> MPTLLRVYIDGPHGMGKTTTTQLLVALGSRDDIVYVPEPMTYWRVLGASETIANIYTTQHRLDQGEISAGDAAVVMTSAQITMGMPYAVTDAVLAPHIGGEAGSSHAPPPALTLIFDRHPIAALLCYPAARYLMGSMTPQAVLAFVALIPPTLPGTNIVLGALPEDRHIDRLAKRQRPGERLDLAMLAAIRRVYGLLANTVRYLQCGGSWREDWGQLSGTAVPPQGAEPQSNAGARPHIGDTLFTLFRAPELLAPNGDLYNVFAWALDVLAKRLRSMHVFILDYDQSPAGCRDALL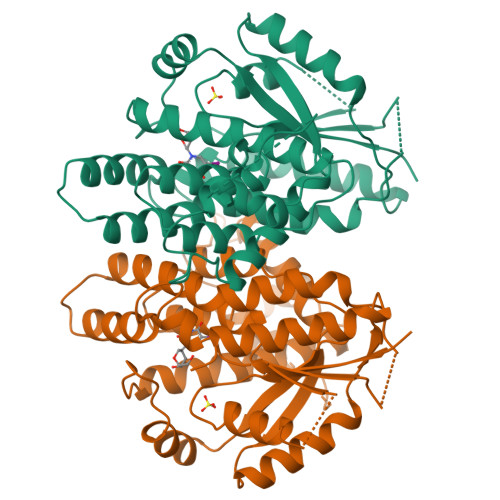QLTSGMVQTHVTTPGSIPTICDLARTFAREMGEAN;> MPTLLRVYIDGPHGMGKTTTTQLLVALGSRDDIVYVPEPMTYWRVLGASETIANIYTTQHRLDQGEISAGDAAVVMTSAQITMGMPYAVTDAVLAPHIGGEAGSSHAPPPALTLIFDRHPIAALLCYPAARYLMGSMTPQAVLAFVALIPPTLPGTNIVLGALPEDRHIDRLAKRQRPGERLDLAMLAAIRRVYGLLANTVRYLQCGGSWREDWGQLSGTAVPPQGAEPQSNAGPRPHIGDTLFTLFRAPELLAPNGDLYNVFAWALDVLAKRLRSMHVFILDYDQSPAGCRDALLQLTSGMVQTHVTTPGSIPTICDLARTFAREMGEAN>[2x]MRRANDPQRREKIIQATLEAVKLYGIHAVTHRKIATLAGVPLGSMTYYFSGIDEL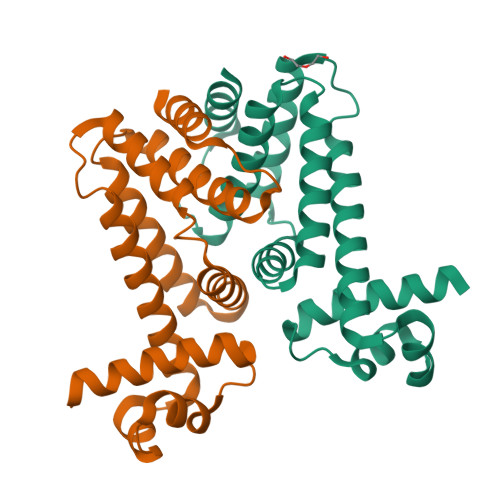LLEAFSSFTEIMSRQYQAFFSDVSDAPGACQAITDMIYSSQVATPDNMELMYQLYALASRKPLLKTVMQNWMQRSQQTLEQWFEPGTARALDAFIEGMTLHFVTDRKPLSREEILRMVERVAG> ITSIWTKGVTPPTNFIEGTDGSHAPYIANQGWYDITKTFNGKDDLLSAAATAGNMLHWWFDQNKNQIEGYLTEHPEKQAIIFNGEQMFDVKEAISTKDRQLDSKLFEYFKEKAFPTLSARRRGVFPDHVIDMFINGYRLSLDNYDKTPVKEGNKDLRGGIFDQVFTRGDQSKLLTNRYNLRTKTINEISQLIKQELIAGKALAISHTYNNIGISHVINLWGADFNSEGNLEAIYVTDSDSNASIGMKKYYVGVNSAGEVAVSSKKIDSEHLGAAALGLYTLSAGQGIWHQTN

In this work, we describe a novel protease of S. canis, termed IdeC (Immunoglobulin G degrading enzyme of S. canis), which may be involved in bacterial immune evasion. We demonstrated IdeC is a cysteine protease that cleaves feline, canine, and human IgG between the hinge and CH2 regions, defining a new virulence determinant for S. canis. The structure of IdeC presents the α/β fold characteristic of the papain superfamily of cysteine proteases, consisting of an α-helix followed by an antiparallel β-sheet comprised of four/five β-strands. The active site, the canonical catalytic triad for papain-like cysteine peptidases (Cys-His-Asn/Gln/Asp/Glu), is situated at the interface and involves residues from both domains.

In an attempt to better understand the structure and function of IdeC, the crystal structure of IdeC (residues 30–339), with a C94S mutation to abolish catalytic activity, was solved at 2.7 Å resolution. The crystals belong to the P32 2 1 space group with one molecule per asymmetric unit. The electron density map allowed perfect modeling of residues 48–339, whereas no electron density was visible for either the N-terminal residues 30–47 or the polyhistidine tag, indicating an inherent flexibility at the N-terminal end of the protein. The catalytic cysteine, Cys94, mutated to a serine in the structure, is located in the L-domain, whereas the catalytic histidine, His262, is found in the R-domain. Asp284 (also in the R-domain) completes the catalytic triad by forming hydrogen bond interactions with His262, orienting its imidazolium ring for the proteolytic reaction. The oxyanion hole is formed by Lys84 and the peptide amide of the catalytic Cys94. Interestingly, a sulfate ion was present at the active site in the structure, with one of its oxygen hydrogen-bonded to the Nz of Lys84 and the amide of Ser94, mimicking the interaction of the scissile carbonyl group of the substrate and the oxyanion hole, which was also observed in other related members of the same family. The remaining oxygens of the sulphate ion establish hydrogen bonds with His262 and the side- hain of Ser94. Residues 254–261 of the IdeC structure form a loop that is equivalent to the prosegment binding loop (PBL) found in other papain superfamily cysteine proteases. The PBL in IdeC, interestingly only eight residues long (in other members of the papain superfamily being around 17–18 residues long), partially obstructs substrate binding and is structured by hydrogen-bond interactions involving the main chains of His253, His262, Ala320, and Ala321 and the side chains of Thr254, Tyr255, His262, Asp284, and Asp286.Variable temperature solution light scattering and/or SAXS experiments have provided important findings about influence of temperature on protein shape or association levels which expand our understanding. Previously, we provided a detailed structural and mechanistic insight of thermophilic l-asparaginase from Pyrococcus furiosus in its full-length (PfA), and a conjoined functional version (cPfA) (domain architecture shown in Supplementary Fig. S1). SAXS and crystal diffraction data analysis brought forth that despite lacking a 19-residue long linker which connects the two domains, namely the N- and C-halves (N-PfA and C-PfA, respectively), cPfA adopts a solution shape and crystalline state that is comparable to wild type full-length protein PfA with improved specific-activity. In conclusion, the findings reported here provide structural evidence in support of temperature induced higher order oligomer formation conferring stability to thermophilic proteins thereby regulating their functioning.

The interactions of P2 with dcPfA forced us to speculate that either this might be non-specific binding or probably another site involved in establishing contact between protein molecules. We thus attempted co-crystallization of cPfA with peptide to further investigate this observation. We successfully co-crystallized cPfA and peptide and the refined structure proved that the P2 retained its binding site thus the interaction was specific. All these interactions were located in a single zone between adjacent protein molecules. This result solved the riddle regarding binding of peptide (P2) at the same site in both peptide-bound dcPfA and cPfA structures.

> MKILLIGMGGTIASVKGENGYEASLSVKEVLDIAGIKDCEDCDFLDLKNVDSTLIQPEDWVDLAETLYKNVKKYDGIIVTHGTDTLAYTSSMISFMLRNPPIPIVFTGSMIPATEENSDAPLNLQTAIKFATSGIRGVYVAFNGKVMLGVRTSKVRTMSRDAFESINYPIIAELRGEDLVVN;> MAVLVIKLIPGLSGDIFRAAVELGYRGIVIEGYGAGGIPYRGSDLLQTIEELSKEIPIVMTTQAMYDGVDLTRYKVGRLALRAGVIPAGDMTKEATVTKLMWILGHTNNVEEIKVLMRKNLVGELRD;> LVVN> GPGSKPFTLPILTIGELSNSRFPVPIDELYTSPNEGVIVQPQNGRSTLDGELLGTTQLVPSNICALRGRINAQVPDDHHQWNLQVTNTNGTPFDPTEDVPAPLGTPDFLANIYGVTSQRNPNNTCRAHDGVLATWSPKFTPKLGSVILGTWEESDLDLNQPTRFTPVGLFNTDHFDQWALPSYSGRLTLNMNLAPSVSPLFPGEQLLFFRSHIPLKGGTSDGAI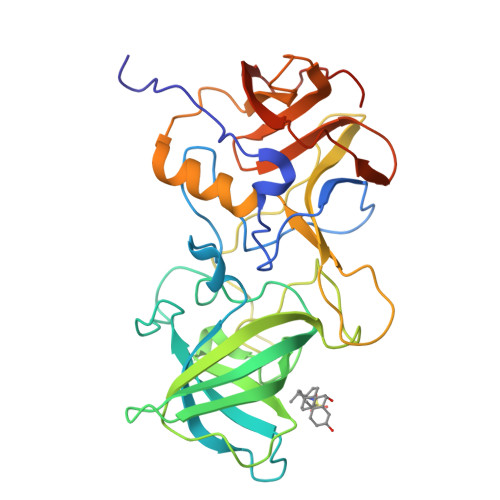DCLLPQEWIQHFYQESAPSPTDVALIRYTNPDTGRVLFEAKLHRQGFITVANSGSRPIVVPPNGYFRFDSWVNQFYSLAPMGTGNGRRRVQ> LPTSNPAQELEARQLGRTTRDDLINGNSASCADVIFIYARGSTETGNLGTLGPSIASNLESAFGKDGVWIQGVGGAYRATLGDNALPRGTSSAAIREMLGLFQQANTKCPDATLIAGGYSQGAALAAASIEDLDSAIRDKIAGTVLFGYTKNLQNRGRIPNYPADRTKVFCKTGDLVCTGSLIVAA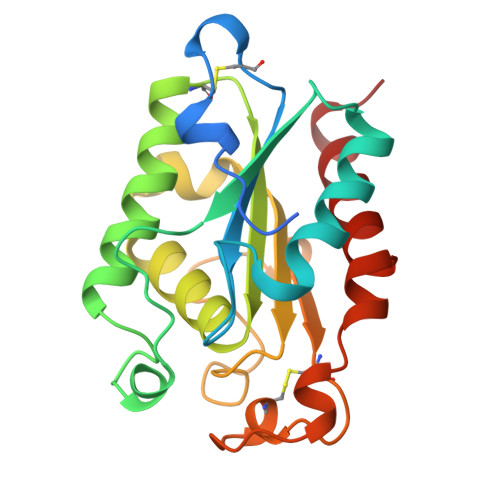PHLAYGPDAEGPAPEFLIEKVRAVRGSA>[2x]MEEIQGYDVEFDPPLESKYECPICLMALREAVQTPCGHRFCKACIIKSIRDAGHKCPVDNEILLENQLFPDNFAKREILSLMVKCPNEGCLHKMELRHLEDHQAHCEFALLEHHHHHH;>[2x]GSHMAGLPRRIIKETQRLLAEPVPGIKAEPDESNARYFHVVIAGPQDSPFEGGTFKLELFLPEEYPMAAPKVRFMTKIYHPNVDKLGRICLDILKDKWSPALQIRT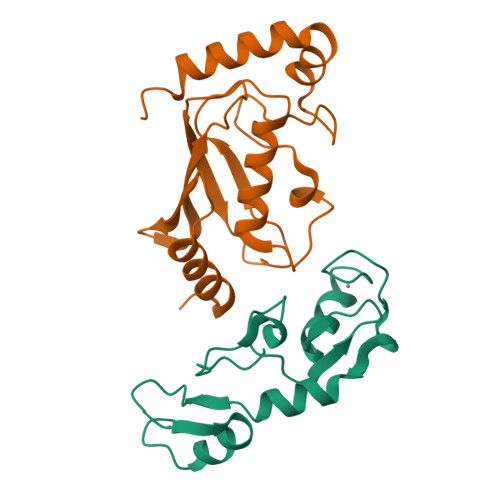VLLSIQALLSAPNPDDPLANDVAEQWKTNEAQAIETARAWTRLYAMNNI>MKNVGFIGWRGMVGSVLMDRMSQENDFENLNPVFFTTSQAGQKAPVFGGKDAGDLKSAFDIEELKKLDIIVTCQGGDYTNEVYPKLKATGWDGYWVDAASALRMKDDAIIVLDPVNQHVISEGLKKGIKTFVGGNCTVSLMLMAIGGLFEKDLVEWISVATYQAASGAGAKNMRELLSQMGLLEQAVSSELKDPASSILDIERKVTAKMRADNFPTDNFGAALGGSLIPWIDKLLPETGQTKDEWKGYAETNKILGLSDNPIPVDGLCVRIGALRCHSQAFTIKLKKDLPLEEIEQIIASHNEWVKVIPNDKEITLRELTPAKVTGTLSVPVGRLRKLAMGPEYLAAFTVGDQLLWGAAEPV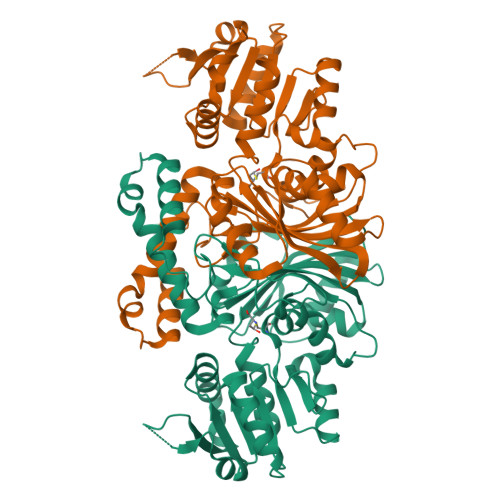RRILKQLVA[2x]>[2x]SVVVISQALPVPTRIPGVADLVGFGNGGVYIIRNSLLIQVVKVINNFGYDAGGWRVEKHVRLLADTTGDNQSDVVGFGENGVWISTNNGNNTFVDPPKMVLANFAYAAGGWRVE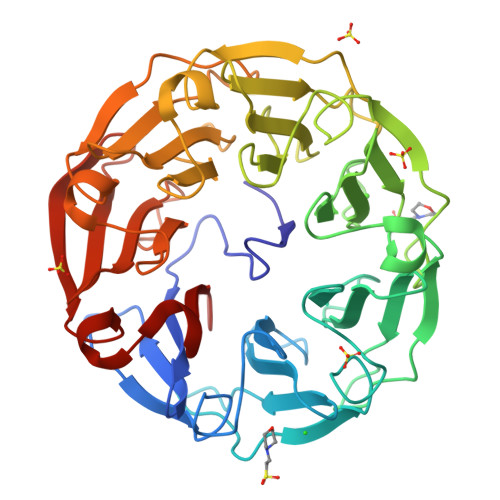KHIRFMADLRKTGRADIVGFGDGGIYISRNNGGGQFAPAQLALNNFGYAQGWRLDRHLRFLADVTGDGLLDVVGFGENQVYIARNSGNGTFQPAQAVVNNFCIGAGGWTISAHPRVVADLTGDRKADILGFGVAGVYTSLNNGNGTFGAVNLVLKDFGVNSGWRVEKHVRCVSSLTNKKVGDIIGFGDAGVYVALNNGNGTFGPVKRVIDNFGYNQGWRVDKHPRFVVDLTGDGCADIVGFGENSVWACMNKGDGTFGPIMKLIDDMTVSKGWTLQKTVRYAANLYL> MSIFTIFISALLVNNFVLSRFLGICPFLGVSKKVETATGMGAAVTFVMALAAIMTFLVERFILIPLNIQYLSTLAFILVIASLVQFVEMVIKKVSPDLYKALGIYLPLITTNCAVLGMAVINSNEKYNLIQSIINSVGAALGFTLALVLLAGIREKMETNEYIPEALKGLPITLVTAGLMAIAFLGFQGLI;> MEGLLFPVLSLGGLGVVFGLLLGYASKKFAVEVDERVPMVRAALPGANCGGCGFAGCDAYADAVVNAGAKPNGCPVGGAACAAKIAEIMGVVVDSSEPKKAYVKCQGTCDKAKEKYEYYGAMTCVDAANIPGAGSKTCGFGCLGLGSCVQVCAFDAIHVENGIAVVDEEACTGCGACVSICPKSVIELTPMSKKVRISCNSHDKGIEVKNACSVGCLSCGLCVRNCPSEAITMVNNLPVIDYDKCTQCGVCVGKCPTKAIVNLNTNVSKEASNN;> MELLTFKNGVHPPHGKHYTENKPIEEYLPKGDIVIPMSQHIGAPAEPIVKKGDRVLVGQKIGEAKGFVSANIHASVSGTVKNVAPVTLFNGVKSTAVIIENDGQYEEIETEKRDYTKLSNEEIINIIKEAGIVGMGGATFPTHVKLAPPPDKNIDSIVVNAAECEPYLTCDHRMMLEKTNEIVEGLKIVLKLFPKATGYIGIEDNKMNAIKAMQEAVKNIANIEVKAVKTKYPQGAEKQLIYAITKREVPSGGLPADAGCIVQNVDTIYEIYNAVVNGKPLTSRVVTVTGDAIKEPKNLRFKIGTSVRELVEAAGGFAEEPLKVISGGPMMGMAMYSLDVPSTKGTSGVLCLTKKVAEIEEESNCINCGKCVQVCPMNLMPTKLATASAVSNLDMFNEFSGRDCIECGCCSFVCPARRHLLQRIRSGKKAVSKKK;> MSETTMYTVSSSPHIRAKDTTQSIMRDVVIALLPATIAGVYFFKLQGLLVILASVLSCVVAEYIWQKASKKKVTVGDYSAVVTGLLLAFNVPASIPLWIPVVGGFFAIIVVKQFFGGLGQNIVNPALAARAFLLASWPVQMTSWTLDGVTTATPLAILKGNEATGAAAPDLMSVFIGHVGGCIGETSALALLIGGAYLFYKHIIDWRIPVSFIGTTFIFTAIAGRGSSPVYELFAGGLMLGAIFMATDYATSPITPLGRIIFGVGCGVITSLIRIFGGYPEGVSYSILVMNLFVPLIERWTAPKIFGKVK;> MGVVSERLYNGIVKENATFVQVLGMCPTLAVTTSAINGIGMGLSATVVLIGSNVVISLLKKVIPDEIRIPAYITVIATLVTVLQFLLQAYLPDLNKSLGIFIPLIVVNCIILGRAEAYANKNSVGASFFDGLGMGLGFTVSLAALGIIREFLGTGKVFGAQITPDAFQPALIMILAPGGFFTLGILMAILNQRKLKKAKAK;> MKKVSSFKLGMVLLLIAAVCGLILGGVNQVTAEPIAIQNKKTLDEANKAILPEASEFAEKTDIKGEGIVLGVTEGKSGSDLKGYTIKVAPKGYAGAIEMMVGVSTEGKVTGIKILNHAETPGLGANATDPKFSGQYANKPAKELKVVKGAASGEDEIVAITGATITSKAVTLGVNEAIKFYDTKLKGGK

Various microbial metabolisms use H+/Na+-translocating ferredoxin:NAD+ reductase (Rnf) either to exergonically oxidize reduced ferredoxin by NAD+ for generating a transmembrane electrochemical potential or reversely to exploit the latter for producing reduced ferredoxin. Electron acceptors are either H+ (E°′ = ‒414 mV)4,5 or NAD+ (E°′ = ‒320 mV). The latter electrogenic NAD+-ferredoxin oxidoreductase reaction is catalyzed by the membrane-spanning multi-subunit complex Rnf (from Rhodobacter N2 fixation metabolism, in which context Rnf was discovered) thereby linking ferredoxin and pyridine nucleotide pools. On this basis, we postulated an electron transfer route between ferredoxin and NAD via eight [4Fe-4S] clusters, one Fe ion and four flavins crossing the cell membrane twice related to the pathway of NADH:ubiquinone reductase. Architecturally, Rnf shows the highest relationship to the electrogenic NADH: ubiquinone reductase complex (Nqr).

For cryo-EM structural analysis, we elaborated a quick four-step purification protocol for the Rnf complex from Clostridium tetanomorphum and integrated the homogeneous and active enzyme into a nanodisc. The overall resolution was determined to 4.27 Å. The Rnf or RnfABCDEG structure consists of membrane-spanning RnfADE (blue A, pink D, sky blue E), extracellular RnfG (brown G), and cytoplasmic RnfB (green B) and RnfC (orange C). The five reliably identified [4Fe-4S] clusters are semi-circularly arranged with distances between 9.0 and 10.5 Å to their corresponding neighbors. The small FdI domain is highly mobile and the density is too noisy for reliable model building and for detecting an iron-sulfur cluster. The Thr153 and Thr164 hydroxy groups form a covalent bond with the phospho groups of FMNRnfD and FMNRnfG, respectively. Most interestingly, RnfG is rotated ca. 35° relative to NqrC27, which changes the position of FMN relative to RnfAE and RnfD as well as their redox cofactors. In the Rnf structure the potential Na+ channel is found in a locked state. In the structurally characterized resting state, the channel is blocked by two hydrophobic layers. In contrast to the wide vestibule with FMN as part of the side wall in Nqr, the equivalent extracellular half-channel in Rnf is occluded by loop 175–187 protruding in a hairpin-shaped fashion from the solvent-exposed outer wall to the isoalloxazine of the central FMNRnfD.>[2x]SLFEL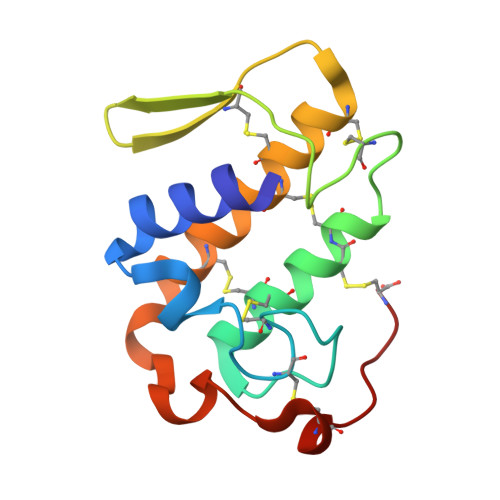GKMILQETGKNPAKSYGAYGCNCGVLGRGGPKDATDRCCYVHKCCYKKLTGCDPKKDRYSYSWKDKTIVCGENNPCLKELCECDKAVAICLRENLGTYNKKYRYHLKPFCKKADPC> MAFQILLNVILAFVWMFLTVSFDGA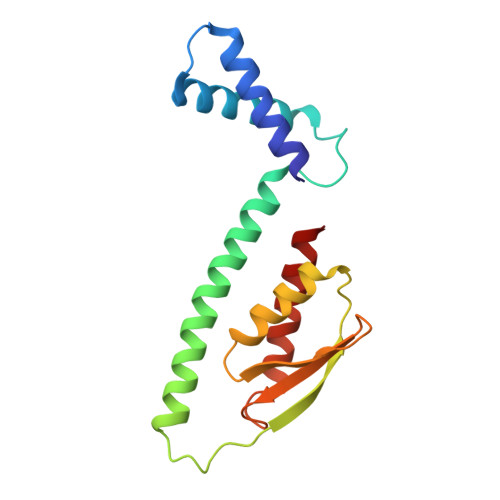SFLVGYMIGLFILFILRRFFHSRFYLVPVFVIIKLLFIFFKELILSNIAVAKVVMQRSLTIQPAIFALPTELKKEWEITVLAMLITLTPGTLVLDVSDDGSTLYIHALNSPDVHEAIESIKQSFEKTIMEVSK>[2x]AIPKVPPGPNITATYGDK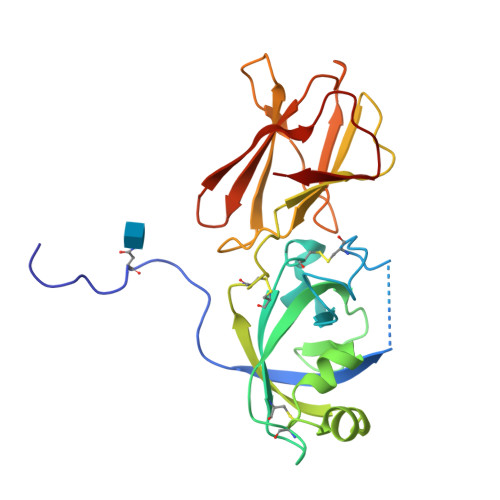WLDAKSTWYGKPTGAGPKDNGGACGYKDVDKPPFSGMTGCGNTPIFKSGRGCGSCFEIKCTKPEACSGEPVVVHITDDNEEPIAPYHFDLSGHAFGAMAKKGDEQKLRSAGELELQFRRVKCKYPEGTKVTFHVEKGSNPNYLALLVKYVNGDGDVVAVDIKEKGKDKWIELKESWGAIWRIDTPDKLTGPFTVRYTTEGGTKTEAEDVIPEGWKADTSYESK> MPFCTSTPEPEAQSTEQSLTCEGQIISGTSVDASDLVTGNEIGEQQLISGDAYVGAQQTGCLPTSPRFNQTGNVQSMGFKNTNQPEQNFAPGEVMPTDFSIQTPARSAQNRITGNDIAPSGRITGPGMLATGLITGTPEFRHAARELVGSPQPMAMAMANRNKAAQAPV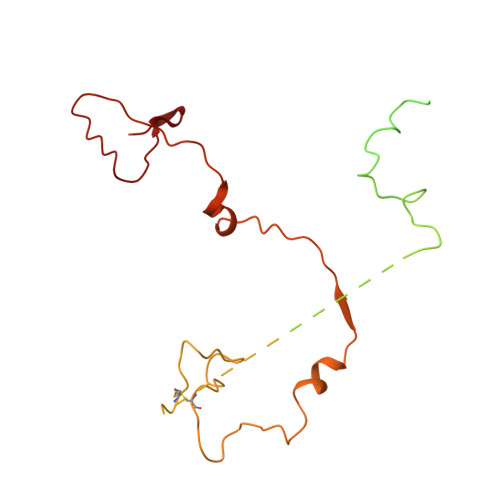VQPEVVATQEKPELVCAPRSDQMDRVSGEGKERCHITGDDWSVNKHITGTAGQWASGRNPSMRGNARVVETSAFANRNVPKPEKPGSKITGSSGNDTQGSLITYSGGARG>[2x]SPDKQMAVLPRRERNRQAAAANPENSRGKGRRGQRGKNRGCVLTAIHLNVTDLGLGYETKEELIFRYCSGSCDAAETTYDKILKNLSRNRRLVSDKVGQACCRPIAFDDDLSFLDDNLVYHILRKHSAKRCGCI;>DRLDCVKASDQCLKEQSCSTKYRTLRQCVAGKETNFSLASGLEAKDECRSAMEALKQKSLYNCRCKRGMKKEKNCLRIYWSMYQSLQGNDLLEDSPYEPVNSRLSDIFRVVPFISDVFQQVEHIPKGNNCLDAAKACNLDDICKKYRSAYITPCTTSVSNDVCNRRKCHKALRQFFDKVPAKHSYGMLFCSCRDIACTERRRQTIVPVCSYEEREKPNCLNLQDSCKTNYICRSRLA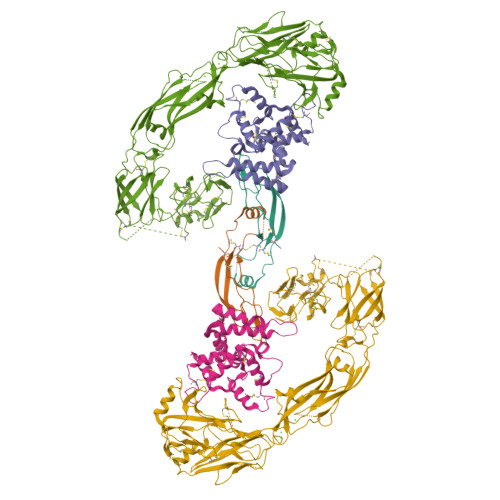DFFTNCQPESRSVSSCLKENYADCLLAYSGLIGTVMTPNYIDSSSLSVAPWCDCSNSGNDLEECLKFLNFFKDNTCLKNAIQAFGNGSDVTVWQPAFPVQTTTATTTTALRVKNKPLGPAGSENEIPTHVLPPCANLQAQKLKSNVSGNTHLCISNGNYEKEGLGGTHHHHHHHH[2x];>LYFSRDAYWEKLYVDQAAGTPLLYVHALRDAPEEVPSFRLGQHLYGTYRTRLHENNWICIQEDTGLLYLNRSLDHSSWEKLSVRNHGFPLLTVYLKVFLSPTSLREGECQWPGCARVYFSFFNTSFPACSSLKPRELCFPETRPSFRIRENRPPGTFHQFRLLPVQFLCPNISVAYRLLEGEGLPFRCAPDSLEVSTRWALDREQREKYELVAVCTVHAGAREEVVMVPFPVTVYDEDDSAPTFPAGVDTASAVVEFKRKEDTVVATLRVFDADVVPASGELVRRYTSTLLPGDTWAQQTFRVEHWPNETSVQANGSFVRATVHDYRLVLNRNLSISENRTMQLAVLVNDSDFQGPGAGVLLLHFNVSVLPVSLHLPSTYSLSVSRRARRFAQIGKVCVENCQAFSGINVQYKLHSSGANCSTLGVVTSAEDTSGILFVNDTKALRRPKCAELHYMVVATDQQTSRQAQAQLLVTVEGSYVAEEAGCPLSCAVSKRRLECEECGGLGSPTGRCEWRQGDGKGITRNFSTCSPSTKTCPDGHCDVVETQDINICPQDCLRGSIVGGHEPGEPRGIKAGYGTCNCFPEEEKCFCEPEDIQDPLCDELCRGTHHHHHHHH[2x]> CVIFPVEIDVSQTIIRDCQVDKQTRE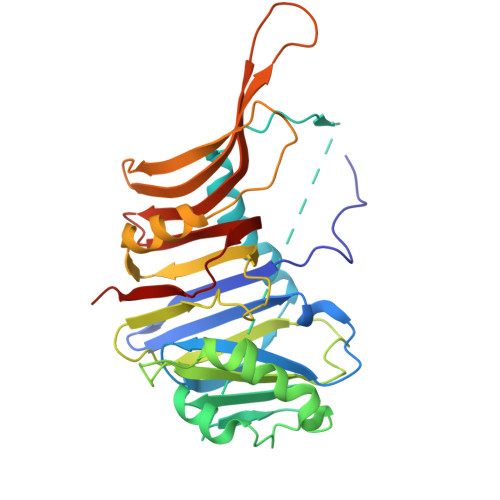LVYINKIMNTQLTKPVLMMFNISGPIRSVTRKNNNLRDRIKSKVDEQFDQLERDYSDQMDGFHDSIKYFKDEHYSVSCQNGSVLKSKFAKILKSHDYTDKKSIEAYEKYCLPKLVDERNDYYVAVCVLKPGFENGSNQVLSFEYNPIGNKVIVPFAHEINDTGLYEYDVVAYVDSVQFDGEQFEEFVQSLILPSSFKNSEKVLYYNEASKNKSMIYKALEFTTESSWGKSEKYNWKIFCNGFIYDKKSKVLYVKLHNVTSALNKNVILNTIK> MKQNKLHYTTMIMTQFPDISIQSVESLGEGFRNYAILVNGDWVFRFPKSQQGADELNKEIQLLPLLVGCVKVNIPQYVYIGKRSDGNPFVGYRKVQGQILGEDGMAVLPDDAKDRLALQLAEFMNELSAFPVETAISAGVPVTNLKNKILLLSEAVEDQV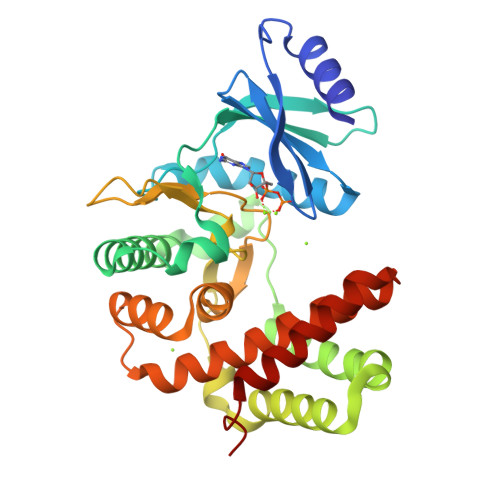FPLLDESLRDYLTLRFQSYMTHPVYTRYTPRLIHGDLSPDHFLTNLNSRQTPLTGIIDFGDAAISDPDYDYVYLLEDCGELFTRQVMAYRGEVDLDTHIRKVSLFVTFDQVSYLLEGLRARDQDWISEGLELLEEDKANNFGANSA> PISPIETVPVKLKPGMDGPKVKQWPLTEEKIKALVEICTEMEKEGKISKIGPENPYNTPVFAIKKKDSTKWRKLVDFRELNKRTQDFWEVQLGIPHPAGLKKNKSVTVLDVGDAYFSVPLDEDFRKYTAFTIPSINNETPGIRYQYNVLPQGWKGSPAIFQSSMTKILEPFRKQNPDIVIYQYMDDLYVGSDLEIGQHRTKIEELRQHLLRWGLTTPDKKHQKEPPFLWMGYELHPDKWTVQPIVLPEKDSWTVNDIQKLVGKLNWASQIYPGIKVRQLCKLLRGTKALTEVIPLTEEAELELAENREILKEPVHGVY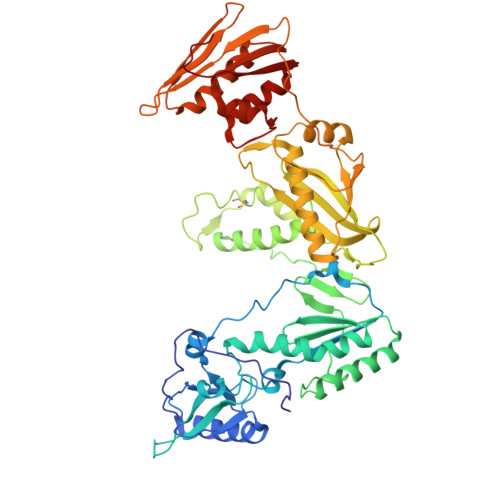YDPSKDLIAEIQKQGQGQWTYQIYQEPFKNLKTGKYARMRGAHTNDVKQLTEAVQKITTESIVIWGKTPKFKLPIQKETWETWWTEYWQATWIPEWEFVNTPPLVKLWYQLEKEPIVGAETFYVDGAANRETKLGKAGYVTNRGRQKVVTLTDTTNQKTELQAIYLALQDSGLEVNIVTDSQYALGIIQAQPDQSESELVNQIIEQLIKKEKVYLAWVPAHKGIG>[2x]TAPSQVLKIRRPDDWHLHLRDGDMLKTVVPYTSEIYGRAIVMPNLAPPVTTVEAAVAYRQRILDAVPAPHDFTPLMTCYLTDSLDPNELERGFNEGVFTAAKLYPANATTNSSHGVTSVDAIMPVLERMEKIGMPLLVHGEVTHADIDIFDREARFIESVMEPLRQRLTALKVVFEHITTKDAADYVRDGNERLAATITPQHLMF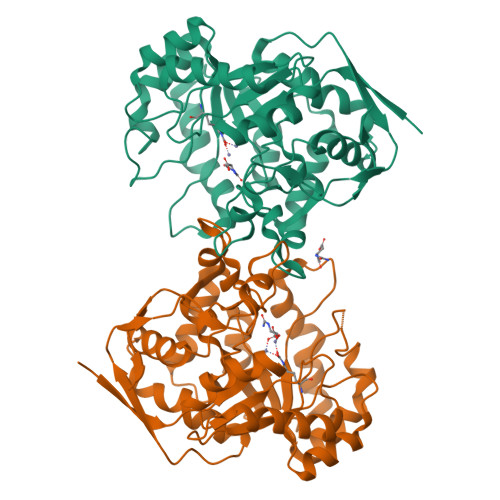NRNHMLVGGVRPHLYCLPILKRNIHQQALRELVASGFQRVFLGTDSAPHARHRKESSCGCAGCFNAPTALGSYATVFEEMNALQHFEAFCSVNGPQFYGLPVNDTFIELVREEQQVAESIALTDDTLVPFLAGETVRWSVKQ> APLAAPSKPIMVTVEEQRSQSVRPGADVTFICTAKSKSPAYTLVWTRLHNGKLPSRAMDFNGILTIRNVQPSDAGTYVCTGSNMFAMD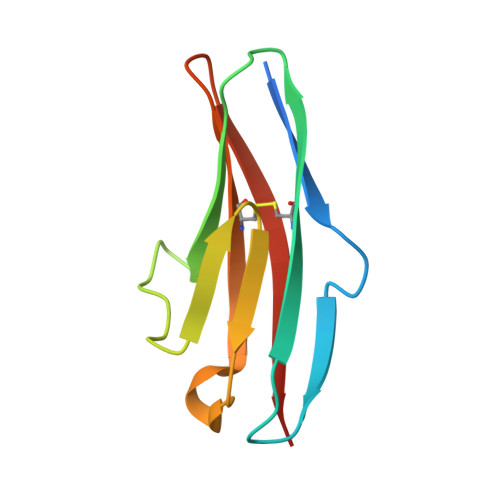QGTATLHVQV>[2x]MSEEQSHADQDAYVADVDGILDVLRAQVLERKPDDIFQFISKSALSLQKDRGAESCDRINCKVKDEQKSRALTIIVFGASGDLAKKKTFPALFDLYCGGLLPPEVNIIGYARTKVDDVEKWKHETLMKYFSNLSERGCHAEDFLKHISYFCGAYDSVDDFKRLDAVIREKENAFKGPEKGGNRLFYLALPPSVFASVCESIHKGAMPQEVGGWVRVIIEKPFGRDTKSSAELSQALEPFFDESQLYRIDHYLGKEMVQNIITTRFANRIFSAVWNASNIACVQITFKETIGTEGRGGYFDNIGIIRDVMQNHLTQILALLAMEKPRSLDAECIRDEKVSVLKCIEPITKENCVLGQYTASADGSIPGYLEDVTVPEGSTCPTFAVMRLNINNDRWAGVPFILKAGKAVEQKYVAIRIQFRDEVHPYGEATQRNELVIRAQPSEAMYVKITTKVPGLSGDLR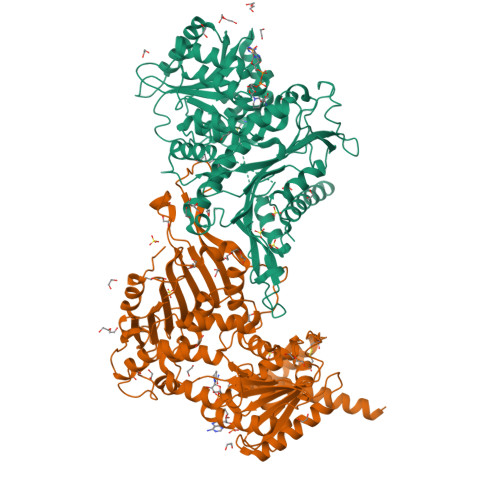QTHQTELDLTYHTRYDVRLPDAYESLINDALLGNSTNFVRKDELDVAWRIFTPLLHQIDSGEIKPIPYQAGTRGPKEADEFIANNGFKHQKGYHWLPSNKL>[2x]M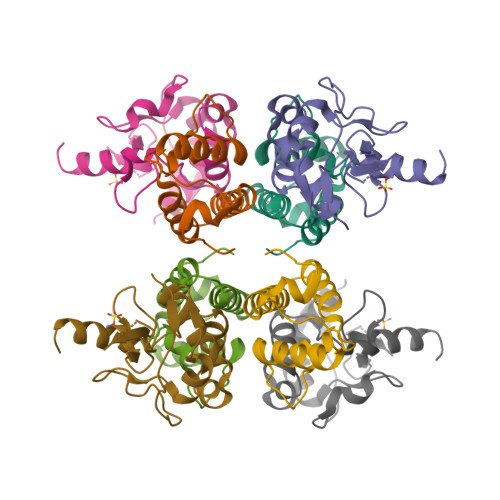ELKNSISDYTEAEFVQLLKEIEKENVAATDDVLDVLLEHFVKITEHPDGTDLIYYPSDNRDDSPEGIVKEIKEWRAANGKPGFKQG;>KRNKPGKATGKGKPVNNKWLNNAGKDLGSPVPDRIANKLRDKEFKSFDDFRKKFWEEVSKDPELSKQFSRNNNDRMKVGKAPKTRTQDVSGKRTSFELHHEKPISQNGGVYDMDAISVVTPKRHIDIHRGK[2x]>MISLADLQRRIETGELSPNAAIAQSHAAIEAREKEVHAFVRHDKSARAQASGPLRGIAVGIKDIIDTANMPTEMGSEIYRGWQPRSDAP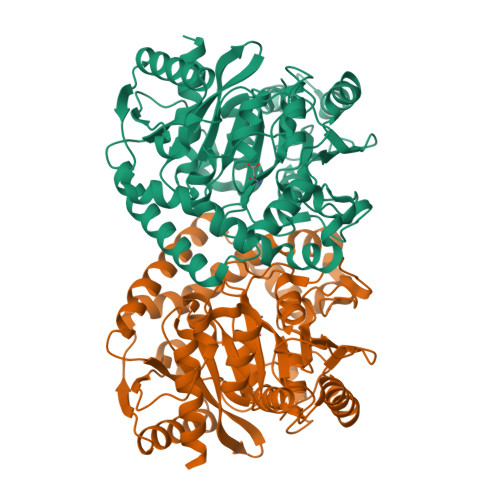VVMMLKRAGATIIGKTTTTAFASRDPTATLNPHNTGHSPGGASSGSAAAVGAGMIPLALGTQTGGSVIRPAAYCGTAAIKPSFRMLPTVGVKCYSWALDTVGLFGARAEDLARGLLAMTGRSEFSGIVPAKAPRIGVVRQEFAGAVEPAAEQGLQAAIKAAERAGASVQAIDLPEAVHEAWRIHPIIQDFEAHRALAWEFSEHHDEIAPMLRASLDATVGLTPKEYDEARRIGRRGRRELGEVFEGVDVLLTYSAPGTAPAKALASTGDPRYNRLWTLMGNPCVNVPVLKVGGLPIGVQVIARFGNDAHALATAWFLEDALAKSG[2x]> GSSMGQPGIINNDLQTLLEVKKSLVTNPQEDDPLRQWNSDNINYCSWTGVTCDNTGLFRVIALNLTGLGLTGSISPWFGRFDNLIHLDLSSNNLVGPIPTALSNLTSLESLFLFSNQLTGEIPSQLGSLVNIRSLRIGDNELVGDIPETLGNLVNLQMLALASCRLTGPIPSQLGRLVRVQSLILQDNYLEGPIPAELGNCSDLTVFTAAENMLNGTIPAELGRLENLEILNLANNSLTGEIPSQLGEMSQLQYLSLMANQLQGLIPKSLADLGNLQTLDLSANNLTGEIPEEFWNMSQLLDLVLANNHLSGSLPKSICSNNTNLEQLVLSGTQLSGEIPVELSKCQSLKQLDLSNNSLAGSIPEALFELVELTDLYLHNNTLEGTLSPSISNLTNLQWLVLYHNNLEGKLPKEISALRKLEVLFLYENRFSGEIPQEIGNCTSLKMIDMFGNHFEGEIPPSIGRLKELNLLHLRQNELVGGLPASLGNCHQLNILDLADNQLSGSIPSSFGFLKGLEQLMLYNNS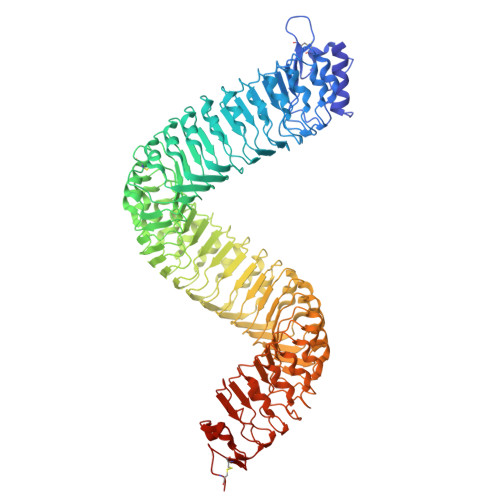LQGNLPDSLISLRNLTRINLSHNRLNGTIHPLCGSSSYLSFDVTNNGFEDEIPLELGNSQNLDRLRLGKNQLTGKIPWTLGKIRELSLLDMSSNALTGTIPLQLVLCKKLTHIDLNNNFLSGPIPPWLGKLSQLGELKLSSNQFVESLPTELFNCTKLLVLSLDGNSLNGSIPQEIGNLGALNVLNLDKNQFSGSLPQAMGKLSKLYELRLSRNSLTGEIPVEIGQLQDLQSALDLSYNNFTGDIPSTIGTLSKLETLDLSHNQLTGEVPGSVGDMKSLGYLNVSFNNLGGKLKKQFSRWPADSFLGNTGLCGSPLSRCNRVRSNNKQQGLENLYFQ>GIDPFTAPAVTQHAPYFKGTAVVNGEFKDLSLDDFKGKYLVLFFYPLDFTFVCPTEIVAFSDKANEFHDVNCEVVAVSVDSHFCHLAWINTPRKNGGLGHMNIALLSDLTKQISRDYGVLLEGSGLALRGLFIIDPNGVIKHLSVNDLPVGRSVEETLRLVKAFQYVETHGEVCPANWTPDSPTIKPSPAASK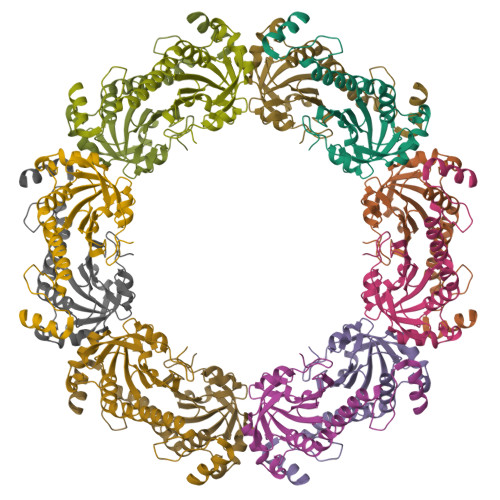EYFQKVNQ[9x]>MVQTSFEHHHHHHSAGENLYFQGAQISMRLYSNRDRPNHLGPLALERLARVDDVVAQPARQPEDGFAASEDSLLGDVEEYARLFTRFLDGPVAPLGDAIPDDPARRAENLKASAYFLDASMVGICRLDPDDRAGDCDPSHTHALVFAVQFGREPEAGEAGAEWIRGTNAARTDMRCAEIAAILSGYVRWMGFPARGHFSGDAQVDLARLAVRAGLARVVDGVLVAPFLRRGFRLGVVTTGYALAADRPLAPEGDLGETAPEVMLGIDGTRPGWEDAEEEKRPLHMGRYPMETIRRVDEPTTLVVRQEIQRVAKRGDFFKRAEAGDLGEKAKQEKKRFPMKHPLALGMQPLIQNMVPLQGTREKLAPTGKGGDLSDPGRNAEAIKALGYYLGADFVGICRAEPWMYYASDEVEGKPIEAYHDYAVVMLIDQGYETMEGASGDDWISASQSMRAYMRGAEIAGVMAAHCRRMGYSARSHSNAHSEVIHNPAILMAGLGEVSRIGDTLLNPFIGPRSKSIVFTTDLPMSVDRPIDFGLQDFCNQCRKCARECPCNAISFGDKVMFNGYEIWKADVEKCTKYRVTQMKGSACGRCMKMCPWNREDTVEGRRLAELSIKVPEARAAIIAMDDALQNGKRNLIKRWWFDLEVIDGVAGAPRMGTNERDLSPDRGDKIGANQKLAMYPPRLQPPPGTTLDAVLPVDRSGGLAEYAAAETPAAARARLKSSAG[3x]

The reductive dehalogenases (RDases) are key enzymes in organohalide respiration, which is performed by a unique subset of bacteria. The RDases are cobalamin-dependent and able to selectively cleave carbon-halogen bonds through reduction. The RDases can be split into two classes: (i) the canonical respiratory dehalogenases, which use a halogenated compound as a final electron acceptor during organohalide respiration and (ii) the catabolic respiratory dehalogenases that occur in the catabolic pathways of non-organohalide respiring bacteria. Structural insight into RDase function is based on two enzymes that have been crystallised, the respiratory perchloroethene (PCE) Sulfurospirillum multivorans reductive dehalogenase (PceA), and the catabolic reductive dehalogenase from Nitratireductor pacificus pht-3B (NpRdhA).

Crystals were obtained in 0.1 M Bis-Tris propane (pH 8.5), 0.2 M sodium nitrate and 20% w/v PEG3350, all with a regular rhombic shape and brown in colour. Crystals belonged to the same C2 space group as NpRdhAC crystals, but yielded a maximum resolution of 1.7Å, with a majority of the data sets diffracting at ~ 2.0 Å (as opposed to NpRdhAC crystals rarely diffracting better than 3.0 Å). The asymmetric unit (AU) contains three monomers that are very similar, with a pairwise alignment rmsd of 0.115–0.148 Å. An overlay of the crystal packing of both NpRdhAC and NpRdhAN reveals the relative position of molecules B and C is particularly affected by the distinct position of the affinity tag, the direct consequence being reduced mobility for these molecules and associated improved diffraction in the case of NpRdhAN. A comparison of the NpRdhAC and NpRdhAN structures by alignment of respective chain A monomers yields an rmsd of 0.148 Å over 614 residues, confirming the distinct position of the hexa-histidine tag has little effect on the protein structure. Furthermore, alignment of active site residues from NpRdhAC and NpRdhAN show excellent agreement with an rmsd of 0.092 Å for the 10 residues selected. A chloride ligand, likely derived from the purification buffer, is modelled as the β–axial ligand at a cobalt-chloride distance of 2.6 Å.> SELIVNVINGPSLGRLGRREPAVYGGTTHDELVALIEREAAELGLKAVVRQSDSEAQLLDWIHQAADAAEPVILNAGGLTHTSVALRDACAELSAPLIEVHISNVHAREEFRRHSYLS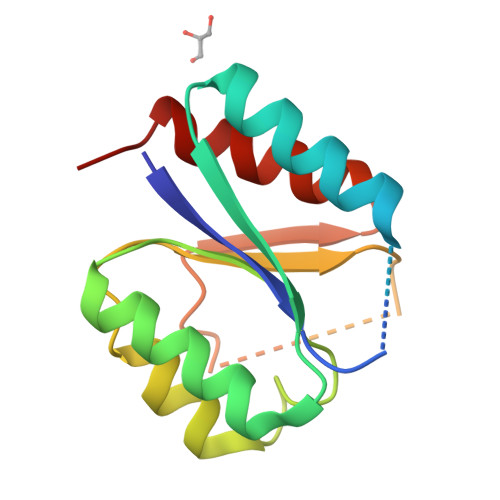PIATGVIVGLGIQGYLLALRYLAEHLGT;>SELIVNVINGPSLGRLGRREPAVYGGTTHDELVALIEREAAELGLKAVVRQSDSEAQLLDWIHQAADAAEPVILNAGGLTHTSVALRDACAELSAPLIEVHISNVHAREEFRRHSYLSPIATGVIVGLGIQGYLLALRYLAEHVGT[3x]>GHMQLLSRRLKLEKEVRNLQEQLITAETARKVEAKNEDKDLQTLIQKWKNAAQQAAEVLFKPMAERIRLAGGVTQSFRIEEGENKGQIQEVRTEFTMSMFLNQFGVPVHLMSFDEENGDWKS[2x];>[2x]MEKSQLESRVHLLEQQKEQLESSLQDALAKLKNRDAKQTVQKHI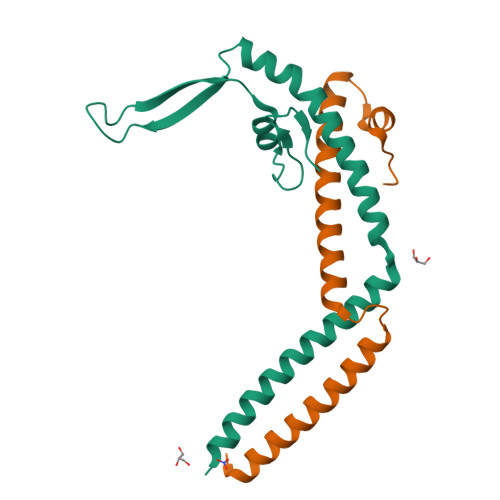DLLHTYNEIRDIALGMIGKVAEHEKCTSVELFDRFGVNGSE>[2x]GVFVFRDETSSSVAPAKLYKALTKDSDTIAQKIDGPIQSIELVEGNGGVGTIKKITANEGDKTSFVLQKVDAIDEANLGYDYSIVGGTGLPESLEKLSFET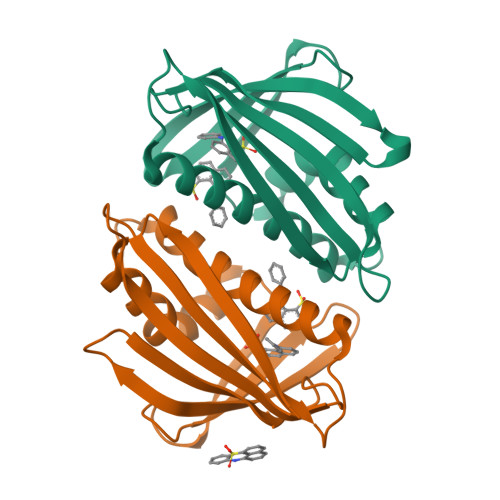KVVAGSGGGSISKVTLKFHTKGDAPLSDAVRDDALAKGAGFFKAIEGYVLANPAEY>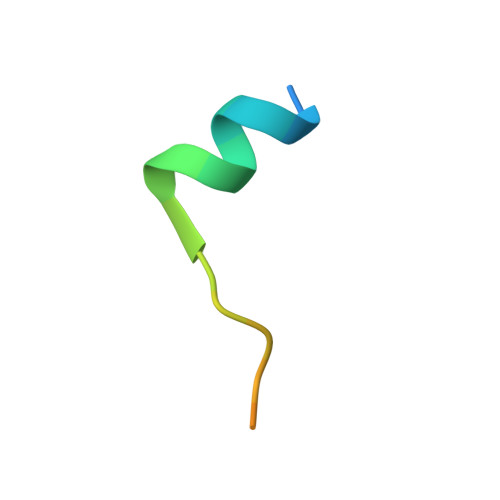 QSEEQVSKNLFGPPLESAFDHED>[2x]MGKTFTVPIVEVTSSFNPATFQSLLIPRDNRPLEVGLLRKVKELLAEVDARTLARHVTKVDCLVARILGVTKEMQTLMGVRWGMELLTLPHGRQLRLDLLERFHTMSIMLAVDILGSTGSAEERAALLHKTIQLAAELRGTMGNMFSFAAVMGALDMAQISRLEQTWVTLRQRHTE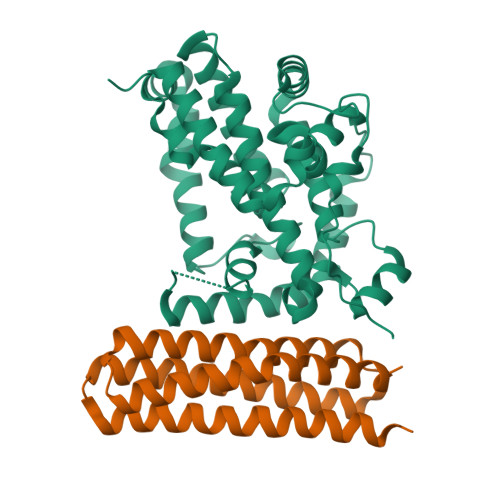GAILYEKKLKPFLKSLNEGKEGPPLSNTTFPHVLPLITLLESDSAPPEGPEPWGSTEHGVEVVLAHLEAARTVAHHGGLYHTNAEVKLQGFQARPELLEVFSTEFQMRLLWGSQGASSSQARRYEKFDKVLTALSHKLEPAVRSSELLEHHHHHH;>MSQDSPDGQYENSEGGWMEDYDYVHLQGKEEFEKTQKELLEKGSITRQGKSQLELQQLKQFERLEQEVSRPIDHDLANWTPAQPLAPGRTGGLGPSDRQLLLFYLEQCEANLTTLTNAVDAFFTAVATNQPPKIFVAHSKFVILSAHKLVFIGDTLSRQAKAADVRSQVTHYSNLLCDLLRGIVATTKAAALQYPSPSAAQDMVERVKELGHSTQQFRRVLGQLAAALE[2x]[(1R)-1,2,3,4-tetrahydroisoquinolin-1-yl]methanol 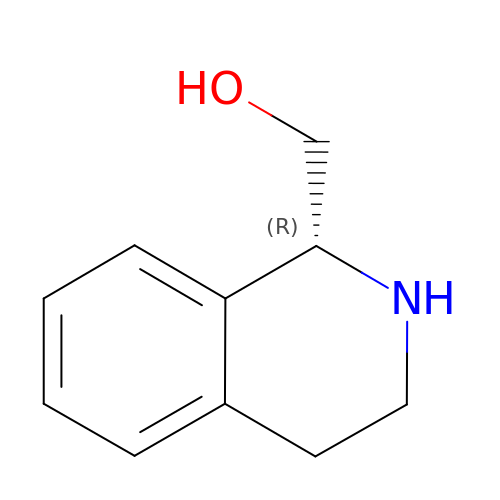| C10 H13 N O | BGGIPVPHBWWEJT-JTQLQIEISA-N> MGSADASTFLNRVCGVSAARLTPCGTGTSTDVVYRAFDIYNEKVAGFAKFLKTNCCRFQEKDEEGNLLDSYFVVKRHTMSNYQHEETIYNLVKDCPAVAVHDFFKFRVDGDMVPHISRQRLTKYTMADLVYALRHFDEGNCDTLKEILVTYNCCDDDYFNKKDWYDFVENPDILRVYANLGERVRQSLLKTVQFCDAMRDAGIVGVLTLDNQDLNGNWYDFGDFVQVAPGCGVPIVDSYYSLLMPILTLTRALAAESHMDADLAKPLIKWDLLKYDFTEERLCLFDRYFKYWDQTYHPNCINCLDDRCILHCANFNVLFSTVFPPTSFGPLVRKIFVDGVPFVVSTGYHFRELGVVHNQDVNLHSSRLSFKELLVYAADPAMHAASGNLLLDKRTTCFSVAALTNNVAFQTVKPGNFNKDFYDFAVSKGFFKEGSSVELKHFFFAQDGNAAISDYDYYRYNLPTMCDIRQLLFVVEVVDKYFDCYDGGCINANQVIVNNLDKSAGFPFNKWGKARLYYDSMSYEDQDALFAYTKRNVIPTITQMNLKYAISAKNRARTVAGVSICSTMTNRQFHQKLLKSIAATRGATVVIGTSKFYGGWHNMLKTVYSDVETPHLMGWDYPKCDRAMPNMLRIMASLVLARKHNTCCNLSHRFYRLANECAQVLSEMVMCGGSLYVKPGGTSSGDATTAYANSVFNICQAVTANVNALLSTDGNKIADKYVRNLQHRLYECLYRNRDVDHEFVDEFYAYLRKHFSMMILSDDAVVCYNSNYAAQGLVASIKNFKAVLYYQNNVFMSEAKCWTETDLTKGPHEFCSQHTMLVKQGDDYVYLPYPDPSRILGAGCFVDDIVKTDGTLMIERFVSLAIDAYPLTKHPNQEYADVFHLYLQYIRKLHDELTGHMLDMYSVMLTNDNTSRYWEPEFYEAMYTPHTVLLVPRGSGHHHHHHAWSHPQFEK;>[2x]AIASEFSSLPSYAAYATAQEAYEQAVANGDSEVVLKKLKKSLNVAKSEFDRDAAMQRKLEKMADQAMTQMYKQARSEDKRAKVTSAMQTMLFTMLRKLDNDALNNIINNARDGCVPLNIIPLTTAAKLMVVVPDYGTYKNTCDGNTFTYASALWEIQQVVDADSKIVQLSEINMDNSPNLAWPLIVTALRANSAVKLQ;> GSKMSDVKCTSVVLLSVLQQLRVESSSKLWAQCVQLHNDILLAKDTTEAFEKMVSLLSVLLSMQGAVDINRLCEEMLDNRATLQ

The nsp12 RNA-dependent RNA polymerase possesses some minimal activity on its own6, but the addition of the nsp7 and nsp8 co-factors greatly stimulates polymerase activity. Though additional viral nsp subunits are likely necessary to carry out the full repertoire of replication and transcription activities, the nsp12-nsp7-nsp8 complex so far represents the minimal complex required for nucleotide polymerization. The SARS-CoV RNA-dependent RNA polymerase resembles a cupped right hand with fingers, palm, and thumb subdomains. Although not previously predicted, the SARS-CoV nsp12 contains two metal-binding sites to which we have assigned zinc atoms.

Here we used cryo-electron microscopy (cryo-EM) to determine the 3.1 Å resolution structure of SARS-CoV nsp12 bound to the nsp7 and nsp8 co-factors. In addition to a structurally conserved polymerase domain, this complex provides the first views of a nidovirus-unique nsp12 N-terminal extension that possesses a kinase-like fold and demonstrates an unexpected binding stoichiometry of nsp7 and nsp8 co-factors. Examination of the cryo-EM map revealed density for a single complex of nsp7-nsp8 heterodimer bound to nsp12 resembling previously determined crystal structures. The nsp7-nsp8 heterodimer binds to nsp12 on the polymerase thumb domain facing the NTP entry channel. Binding in this position sandwiches the nsp12 polymerase index finger loop between nsp7-nsp8 and the polymerase thumb domain. The index finger–thumb interaction site also forms the nsp7-nsp8 heterodimer-binding site, with most of the contacts made between nsp12 and nsp7. 98–126 appears to adopt a conformation unique from those previously observed and involves a refolding of loops and a helical region to participate in interactions with nsp12 and precludes an interaction with nsp7. The role of nsp7 and nsp8 heterodimers appears to be the stabilization of nsp12 regions involved in RNA binding while a second subunit of nsp8 also plays a crucial role in polymerase activity possibly by extending the template RNA-binding surface.>[4x]MAKILCVLYDDPITGYPKSYARADVPKIDHYPGGQTAPTPKQIDFTPGELLGSVSGELGLRKYLEGLGHTLVVTSDKEGEDSVFERELPDAEIVISQPFWPAYLTPERIAKAKKLKLAVTAGIGSDHVDLEAAIKNGITVAEV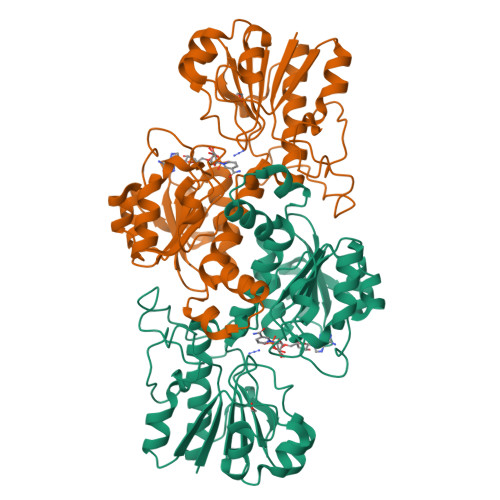TYSNSISVSEHVVMMILSLVRNYIPSYQWVIKGGWNIADCVERSYDLEAMHVGTVAAGRIGLAVLKRLKPFDVKLHYFDQHRLPESVENELGLTYHPSVEDMVKVCDVVTINAPLHPGTLDLFNDELISKMKRGAYLVNTARGKICNRDAVVRALESGQLAGYAGDVWFPQPAPKDHPWRTMPHHGMTPHISGTSLSAQARYAAGTREILECWFEERPIREEYLIVDGGKLAGTGAHSYTVSK>[4x]MTSASSPPAFRLETSDGDEEGNAEVNKGKQEPPPMESPFQREDRNSSPQIKVNLNFIKRPPKNTSAPSQQEPDRFDRDRLFSVVSRGVPEELTGLLEYLRWNSKYLTDSAYTEGSTGKTCLMKAVLNLQDGVNACIMPLLQIDKDSGNPKPLVNAQCTDEFYQGHSALHIAIEKRSLQCVKLLVENGADVHLRACGRFFQKHQGTCFYFGELPLSLAACTKQWDVVTYLLENPHQPASLEATDSLGNTVLHALVMIADNSPENSALVIHMYDGLLQMGARLCPTVQLEEISNHQGLTPLKLAAKEGKIEIFRHILQREFSGPYQPLSRKFTEWCYGPVRVSLYDLSSVDSWEKNSVLEIIAFHCKSPNRHRMVVLEPLNKLLQEKWDRLVSRFFFNFACYLVYMFIFTVVAYHQPSLDQPAIPSSKATFGESMLLLGHILILLGGIYLLLGQLWYFWRRRLFIWISFMDSYFEILFLLQALLTVLSQVLRFMETEWYLPLLVLSLVLGWLNLLYYTRGFQHTGIYSVMIQKVILRDLLRFLLVYLVFLFGFAVALVSLSREARSPKAPEDNNSTVTEQPTVGQEEEPAPYRSILDASLELFKFTIGMGELAFQEQLRFRGVVLLLLLAYVLLTYVLLLNMLIALMSETVNHVADNSWSIWKLQKAISVLEMENGYWWCRRKKHREGRLLKVGTRGDGTPDERWCFRVEEVNWAAWEKTLPTLSEDPSGPGITGNKKNPTSKPGKNSASEEDHLPLQVLQSPTETSQVAPA

TRPV2 is a member of the TRPV subfamily and shares ∼50% sequence identity with TRPV1. While heterologously expressed and endogenous TRPV1 localizes to the plasma membrane and is activated by noxious heat and endogenous and exogenous vanilloids, heterologously expressed TRPV2 predominantly localizes to intracellular membranes. In addition, TRPV2 does not respond to heat or vanilloids in vivo812. In heterologous expression systems, TRPV2 activity was shown to be increased by exogenous small molecules such as 2-aminoethoxydiphenyl borate (2-APB) and probenecid, and blocked by ruthenium red and Gd3715.

Here we report the structure of full-length rat TRPV2 at ∼5 Å resolution determined by cryo-EM single particle reconstruction. Based on the cryo-EM map, we are able to build models for all transmembrane (TM) helices (S1–S6), the pore helix, the selectivity filter, the N-terminal linker and a portion of the C terminus of the channel using the previously published TRPV1 atomic models as homology models. All six N-terminal ankyrin repeats of the ankyrin repeat domain (ARD) are clearly resolved, suggesting that the ARD is a rigid, stable domain in full-length TRPV2. Despite the expression of full-length TRPV2, density accounting for the first 73 residues of the N terminus (Met 1–Asp 73), the S1–S2 linker (Ile 422–Gly 430), the pore turret (Glu 561–Leu 594) and the last 46 residues of the C terminus (Glu 716–Pro 761) are not apparent in the cryo-EM map (grey), suggesting that these regions are flexible or disordered. Like TRPV1 and TRPA1, the pore of apo-TRPV2 consists of two constrictions or gates: an upper gate resides at the selectivity filter in the outer pore region of the channel and a lower gate is comprised of the distal end of S6. A more detailed structural analysis of the apo-TRPV2 pore domain unexpectedly revealed that the upper and lower constrictions are wider than the homologous sites of TRPV1 (Gly 643 and Ile 679) in the absence of ligand (apo-TRPV1) with distances of 12.4 Å and 16.1 Å when measured Cα–Cα at the upper and lower constrictions, respectively. The upper gate of apo-TRPV2 is wider than the closed upper gate of TRPV1 (apo- and capsaicin–TRPV1), as well as the open upper gate of TRPV1 (RTX/DkTx–TRPV1). In addition, the lower gate of apo-TRPV2 has a larger Cα–Cα distance compared with TRPV1 in all states, including the open lower gate in RTX/DkTx–TRPV1 (14.4 Å). These results suggest that the TRPV2 channel can accommodate partially hydrated Ca2+, Na+ and K+ ions, as well as large organic cations in the apo state. Our analysis reveals that in the absence of ligand, full-length rat TRPV2 contains wider upper and lower gates compared with the ‘minimal' rat TRPV1 and truncated rabbit TRPV2.> MSADAQSFLNRVCGVSAARLTPCGTGTSTDVVYRAFDIYNDKVAGFAKFLKTNCCRFQEKDEDDNLIDSYFVVKRHTFSNYQHEETIYNLLKDCPAVAKHDFFKFRIDGDMVPHISRQRLTKYTMADLVYALRHFDEGNCDTLKEILVTYNCCDDDYFNKKDWYDFVENPDILRVYANLGERVRQALLKTVQFCDAMRNAGIVGVLTLDNQDLNGNWYDFGDFIQTTPGSGVPVVDSYYSLLMPILTLTRALTAESHVDTDLTKPYIKWDLLKYDFTEERLKLFDRYFKYWDQTYHPNCVNCLDDRCILHCANFNVLFSTVFPPTSFGPLVRKIFVDGVPFVVSTGYHFRELGVVHNQDVNLHSSRLSFKELLVYAADPAMHAASGNLLLDKRTTCFSVAALTNNVAFQTVKPGNFNKDFYDFAVSKGFFKEGSSVELKHFFFAQDGNAAISDYDYYRYNLPTMCDIRQLLFVVEVVDKYFDCYDGGCINANQVIVNNLDKSAGFPFNKWGKARLYYDS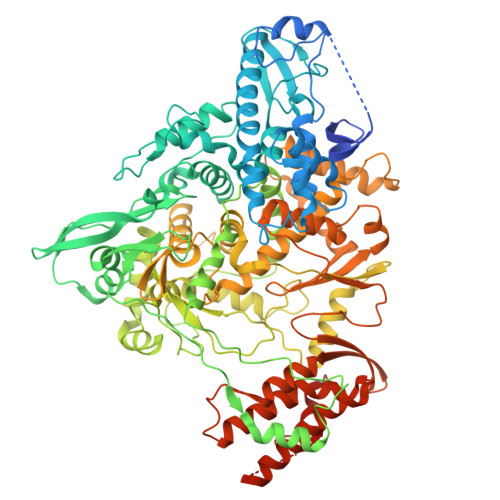MSYEDQDALFAYTKRNVIPTITQMNLKYAISAKNRARTVAGVSICSTMTNRQFHQKLLKSIAATRGATVVIGTSKFYGGWHNMLKTVYSDVENPHLMGWDYPKCDRAMPNMLRIMASLVLARKHTTCCSLSHRFYRLANECAQVLSEMVMCGGSLYVKPGGTSSGDATTAYANSVFNICQAVTANVNALLSTDGNKIADKYVRNLQHRLYECLYRNRDVDTDFVNEFYAYLRKHFSMMILSDDAVVCFNSTYASQGLVASIKNFKSVLYYQNNVFMSEAKCWTETDLTKGPHEFCSQHTMLVKQGDDYVYLPYPDPSRILGAGCFVDDIVKTDGTLMIERFVSLAIDAYPLTKHPNQEYADVFHLYLQYIRKLHDELTGHMLDMYSVMLTNDNTSRYWEPEFYEAMYTPHTVLQGGSENLYFQGHHHHHHHH> CHREPPPETPDINQLPPSILLKIFSNLSLDERCLSASLVCKYWRDLCLDFQFWKQLDLSSRQQVTDELLEKIASRSQNIIEINISDCRSMSDNGVCVLAFKCPGLLRYTAYRCKQLSDTSIIAVASHCPLLQKVHVGNQDKLTDEGLKQLGSKCRELKDIHFGQCYKISDEGMIVIAKGCLKLQRIYMQENKLVTDQSVKAFAEHCPELQYVGFMGCSVTSKGVIH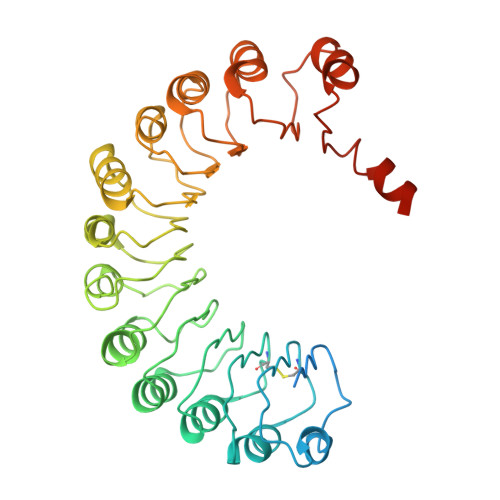LTKLRNLSSLDLRHITELDNETVMEIVKRCKNLSSLNLCLNWIINDRCVEVIAKEGQNLKELYLVSCKITDYALIAIGRYSMTIETVDVGWCKEITDQGATLIAQSSKSLRYLGLMRCDKVNEVTVEQLVQQYPHITFSTVLQDCKRTLERAYQMGWTPNMSAASS2-[4-[[3-[3-(phenylmethyl)-8-(trifluoromethyl)quinolin-4-yl]phenoxy]methyl]phenyl]ethanoic 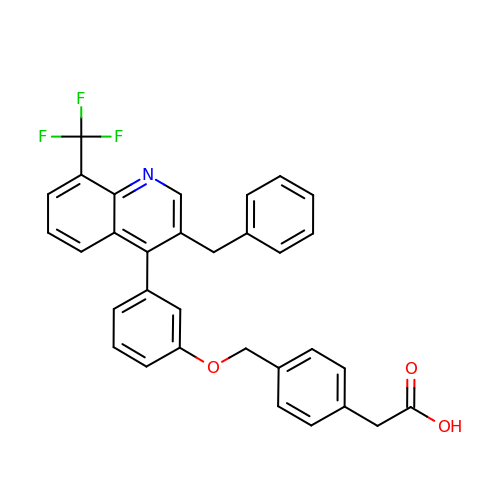acid | C32 H24 F3 N O3 | VXHRQVMQVYQGQG-UHFFFAOYSA-N> DRHRIEEKR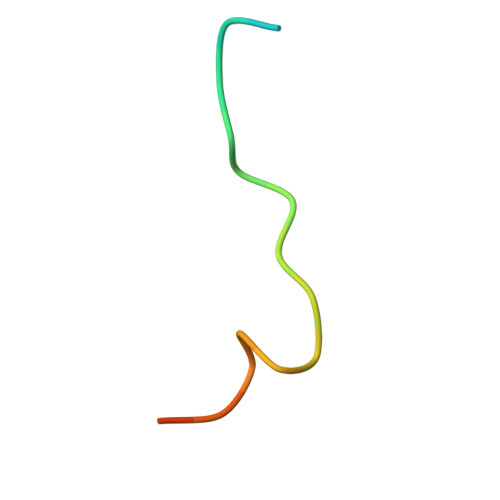KRTYETFKSIMKK The reaction catalysed by TK involves the transfer of a γ-phosphoryl moiety from ATP to 2'deoxy-thymidine (dThd) to produce thymidine 5'-monophosphate (dTMP). TKs of type 2 include those from poxviridae such as vaccinia virus (VV) and variola virus,, as well as from human hTK, (human type II thymidine kinase 1) and mouse. Type 2 TKs have a smaller polypeptide chain compared to type 1, being of ~25 KDa but form homotetramers. They are sensitive to the feedback inhibitors dTDP or dTTP, which are generated at the end of the metabolic pathway.

We report here for the first time, the structure of VVTK, one of the smallest type 2 TKs known, in complex with dTTP at 3.1 Å resolution. The four VVTK subunits within the tetramer are identical apart from a flexible loop (residues 40 to 60) situated on the surface. As found in other type 2 TKs, VVTK has a central α/β domain structure consisting of six parallel β-strands surrounded by helices. Above the α/β domain, a zinc-binding domain is present, the latter belongs to the structural zinc-binding class. Although no zinc was added during purification or crystallization, the metal is present in the structure and coordinated to four cysteines. The phosphates of dTTP bind to the α/β domain, whereas the thymine base and the deoxyribose bind between the lasso domain and the α/β domain. The thymine moiety is bound to the backbone of the protein via residues Phe-113, Ile-157 and 159. In the VVTK active site Ser-148 replaces the equivalent residue in hTK, Thr-163, a serine being also present in UuTK. Asp-43 and Arg-45 are only observed in the VVTK subunit D, they are disordered in the other three subunits, indicating the flexible nature of this loop. The Ser18Thr mutant shows a greater enhancement of enzyme activity (~3.8-fold) than does Thr19Ser and indeed in our structure, Ser-18 forms hydrogen bonds via its main-chain nitrogen to a γ-phosphate oxygen and via its side-chain oxygen to the magnesium and a γ-phosphate oxygen.

>MNGGHIQLIIGPMFSGKSTELIRRVRRYQIAQYKCVTIKYSNDNRYGTGLWTHDKNNFEALEATKLCDVLQSITDFSVIGIDEGQFFPDIVEFCERMANEGKIVIVAALDGTFQRKPFNNILNLLILSEMVVKLTAVCMKCFKEASFSKRLGEETEIEIIGGNDMYQSVCRKCYVGS[4x]> SNDNIELVDFQNIMFYGDAEVGDNQQPFTFILDTGSANLWVPSVKCTTAGCLTKHLYDSSKSRTYEKDGTKVEMNYVSGTVSGFFSKDLVTVGNLSLPYKFIEVIDTNGFEPTYTASTFDGILGLGWKDLSIGSVDPIVVELKNQNKIENALFTFYLPVHDKHTGFLTIGGIEERFYEGPLTYEKLNHDLYWQITLDAHVGNIMLEKANCIVDSGTSAITVPT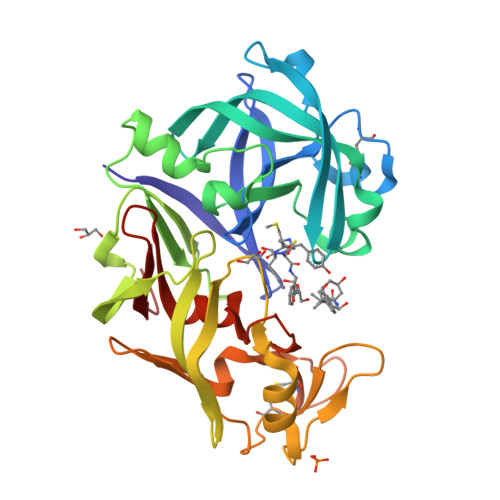DFLNKMLQNLDVIKVPFLPFYVTLCNNSKLPTFEFTSENGKYTLEPEYYLQHIEDVGPGLCMLNIIGLDFPVPTFILGDPFMRKYFTVFDYDNQSVGIALAKKNL>GFGNGNGFG[2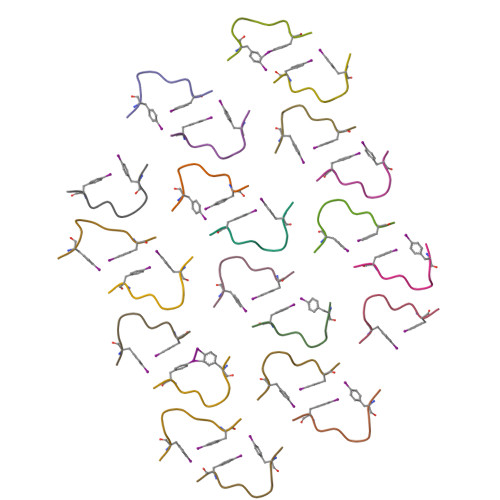2x]>[2x]GMMTDEARAKLAAIPMLAGYTGPLERLGGLTNLVFRAGDLCLRIPGKGTEEYINRANEAVAAREAAKAGVSPEVLHVDPATGVMVTRYIAGAQTMSPEKFKTRPGSPARAGEAFRKLHGSGAVFPFRFELFAMIDDYLKVLSTKNVTLPAGYHDVVREAGGVRSALAAHPLPLAACHCDPLCENFLDTGERMWIVDWEYSGMNDPLWDL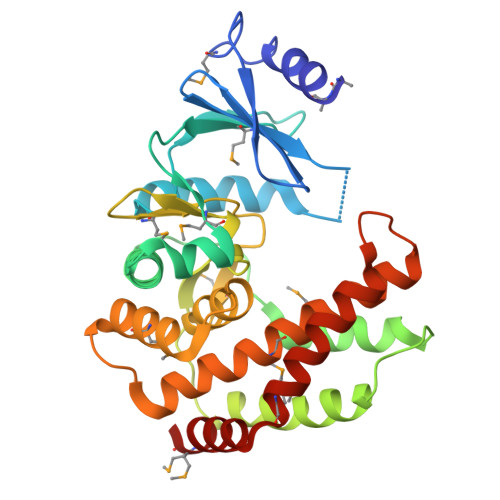GDLSVEGKFNANQDEELMRAYFGGEARPAERGRVVIYKAMCDLLWTLWGLIQLANDNPVDDFRAYADGRFARCKALMETPEFSRHLAAVRMG> ANVPTGVQLAEKQVLVRNNGSEPQSLDPHKIEGVPESNISRDLLEGLVINDPNGNIVPGAAESWDNKDFKVWTFNIRKDAKWSNGDPVTAQDFVYSWQRLADPKTVSPYASYLQYAHLTNIDDIITGKAAPDTLGVKALDDHTLEVTLSEPVPYLDKLLAHPLMSPVNKTVVEKFGEKWTQPQNFVGNGAYKLKDWIVNERIVLERSPTYWDNAKTVINQVTYLPISSEVTDVNRYRSGEIDMTYNNMPIELFQKLKKEIPDQVHVDPYLCTYYYEINNQKAPFTDARVREALKLGMDRDIIVNKVKNQGDLPAYGFTPPYTSGAELTPPEWFSWTQEKRNEVAKKLLAEAGYTKDNPLKFSLLYNTSDLHKKLAIAAASIWKKNLGVDVKLENQEWKTFLDTRHQGTYDVARAAWCADYNEPSSFLNMMLSNSSNNTTHYKSSVFDKLIEDTLKVKSEKERADLYQQAEIQLDKDSAIVPVFYYV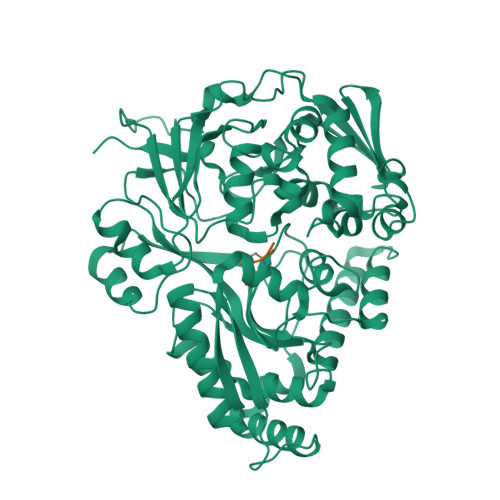SARLVKPYVGGYTGKDPLDNMHVKDLYIIKQ;> KKK> MGSDKIHHHHHHENLYFQGMLHHVEINVDHLEESIAFWDWLLGELGYEDYQSWSRGKSYKHGKTYLVFVQTEDRFQTPTFHRKRTGLNHLAFHA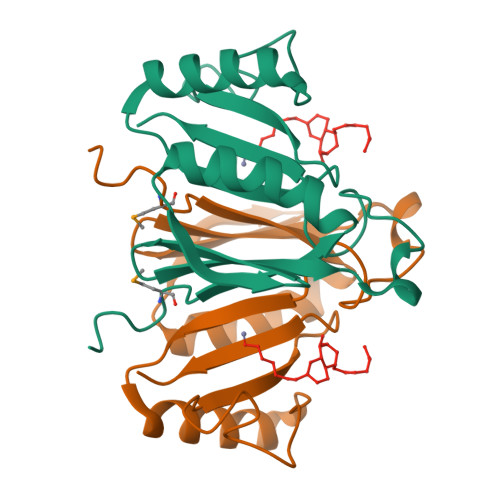ASREKVDELTQKLKERGDPILYEDRHPFAGGPNHYAVFCEDPNRIKVEIVAP> MSPEQLGMIEKLVAAQQQCNRRSFSDRLRVTPWPMAPDPHSREARQQRFAHFTELAIVSVQEIVDFAKQLPGFLQLSREDQIALLKTSAIEVMLLETSRRYNPGSESITFLKDFSYNREDFAKAGLQVEFINPIFEFSRAMNELQLNDAEFALLIAISIFSADRPNVQDQLQVE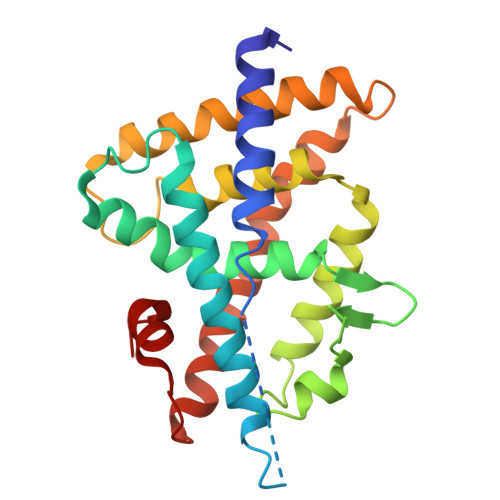RLQHTYVEALHAYVSIHHPHDRLMFPRMLMKLVSLRTLSSVHSEQVFALRLQDKKLPPLLSEIWDVHE>MAEPQPPSGGLTDEAALSCCSDADPSTKDFLLQQTMLRVKDPKKSLDFYTRVLGMTLIQKCDFPIMKFSLYFLAYEDKNDIPKEKDEKIAWALSRKATLELTHNWGTEDDETQSYHNGNSDPRGFGHIGIAVPDVYSACKRFEEL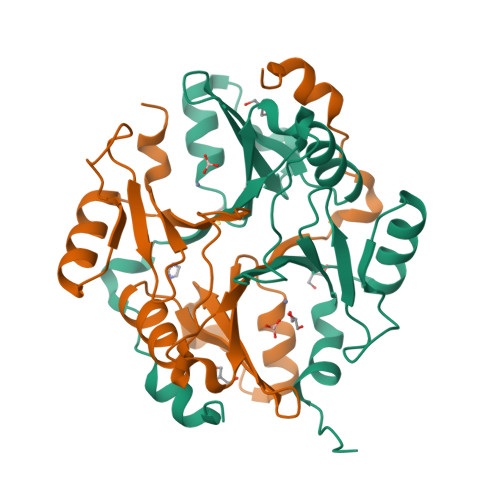GVKFVKKPDDGKMKGLAFIQDPDGYWIEILNPNKMATLMLEHHHHHH[2x]>APASLLPPAPEHSPPSSPLTQPPEGPKFPRVKNWEVGSITYDTLSAQAQQDGPCTPRRCLGSLVFPRKLQGRPSPGPPAPEQLLSQARDFINQYYSSIKRSGSQAHEQRLQEVEAEVAATGTYQLRESELVFGAKQAWRNAPRCVGRIQWGKLQVFDARDCRSAQEMFTYICNHIKYATNRGNLRSAITVFPQRCPGRGDFRIWNSQLVRYAGYRQQDGSVRGDPANVEITELCIQHGWTPGNGRFDVLPLLLQAPDEPPELFLLPPELVLEVPLEHPTLEWFAALGLRWYALPAVSNMLLEIGGLEFPAAPFSGWYMSTEIGTRNLCDNHRYNILEDVAVCMDLDTRTTSSLWKDKAAVEINVAVLHSYQLAKVTIVDHHAATASFMKHLENEQKARGGCPADWAWIVPPISGSLTPVFHQEMVNYFLSPAFRYQPDPW[4x]

Nitric oxide (NO) is an important signaling molecule critical in the cardiovascular, neuronal, and immune systems. The enzyme responsible for generating NO is nitric oxide synthase (NOS), a P450-like heme thiolate enzyme that oxidizes l-arginine to NO and L-citrulline. Humans and other mammals express three different NOS isoforms: endothelial NOS (eNOS), neuronal NOS (nNOS), and inducible NOS (iNOS). nNOS is an important therapeutic target since the overproduction of NO by nNOS in the brain is associated with a number of neurodegenerative diseases. Thus, nNOS is an attractive target for therapeutic intervention. In our efforts to develop inhibitors selective for neuronal nitric oxide synthase (nNOS) over endothelial nitric oxide synthase (eNOS), we found that nNOS can undergo conformational changes in response to inhibitor binding that does not readily occur in eNOS. Here, we used a combination of crystallography, mutagenesis, and computational methods to better understand the structural basis for these differences in NOS inhibitor binding.

First, we examined the sequence variations between hnNOS and heNOS in the region Ile598–Ile611, where the backbone changes occur in hnNOS. The position of Asn606 in hnNOS corresponds to Pro370 in heNOS. The rigidity of the Pro residue could be one reason that heNOS resists undergoing backbone changes upon inhibitor binding. Two reverse mutations were made, hnNOS N606P and heNOS P370N, to test this idea. However, the crystal structure of heNOS P370N bound with 4 revealed that the inhibitor still binds only at the active site while BH4 is undisturbed, just as in the wild-type heNOS-4 complex. Since the single residue variation between Asn606 in hnNOS and Pro370 in heNOS does not appear to be the reason for the backbone dynamic differences, we next analyzed the connection between BH4 binding and the structural changes induced by inhibitor binding in this region. Our mutagenesis results showed that this is not the case.> DVFFSHWTSKYKERNPTEIAYSEDIERIIDSLVTDEITKEEIIHFLFGNFCFHIETMNDQHIADKFKGYQSSCINLKIEPKVDLADLKDHLIQKQQIWESLYGKHLEKIMLRIREKKKKEKEIPDITTAFNQNAAEYEEKYPNCFTNDLSETKTNFSMTWSPSFEKIELSSEVDYNNAIINKFRESFKSSSRVIYNSPYSCINNQTNKARDITNLVRLCLTELSCDTTKMEKQELEDEIDINTGSIKVERTKKSKEWNKQGSCLTRNKNEFCMKETGRENKTIYFKGLAVMNIGMSSKKRILKKEEIKERISKGLEYDTSERQADPNDDYSSIDMSSLTHMKKLIRHDNEDSLSWCERIKDSLFVLHNGDIREEGKITSVYNNYAKNPECLYIQDSVLKTELETCKKINKLCNDLAIYHYSEDMMQFSKGLMVADRYMTKESFKILTTANTSMMLLAFKGDGMNTGGSGVPYIALHIVDEDMSDQFNICYTKEIYSYFRNGSNYIYIMRPQRLNQVRLLSLFKTPSKVPVCFAQFSKKANEMEKWLKNKDIEKVNVFSMTMTVKQILINIVFSSVMIGTVTKLSRMGIFDFMRYAGFLPLSDYSNIKEYIRDKFDPDITNVADIYFVNGIKKLLFRMEDLNLSTNAKPVVVDHENDIIGGITDLNIKCPITGSTLLTLEDLYNNVYLAIYMMPKSLHNHVHNLTSLLNVPAEWELKFRKELGFNIFEDIYPKKAMFDDKDLFSINGALNVKALSDYYLGNIENVGLMRSEIENKEDFLSPCYKISTLKSSKKCSQSNIISTDEIIECLQNAKIQDIENWKGNNLAIIKGLIRTYNEEKNRLVEFFEDNCVNSLYLVEKLKEIINSGSITVGKSVTSKFIRNNHPLTVETYLKTKLYYRNNVTVLKSKKVSEELYDLVKQFHNMMEIDLDSVMNLGKGTEGKKHTFLQMLEFVMSKAKNVTGSVDFLVSVFEKMQRTKTDREIYLMSMKVKMMLYFIEHTFKHVAQSDPSEAISISGDNKIRALSTLSLDTITSYNDILNKNSKKSRLAFLSADQSKWSASDLTYKYVLAIILNPILTTGEASLMIECILMYVKLKKVCIPTDIFLNLRKAQGTFGQNETAIGLLTKGLTTNTYPVSMNWLQGNLNYLSSVYHSCAMKAYHKTLECYKDCDFQTRWIVHSDDNATSLIASGEVDKMLTDFSSSSLPEMLFRSIEAHFKSFCITLNPKKSYASSSEVEFISERIVNGAIIPLYCRHLANCCTESSHISYFDDLMSLSIHVTMLLRKGCPNEVIPFAYGA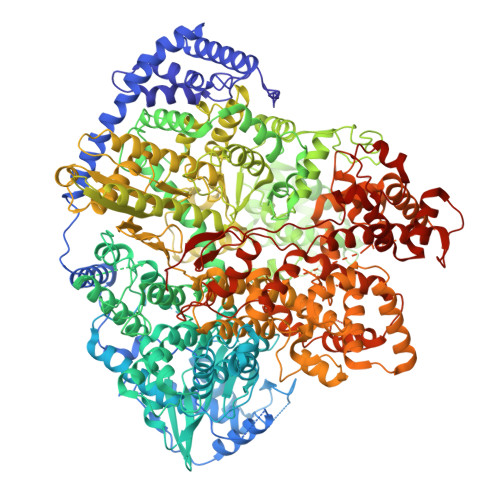VQVQALSIYSMLPGEVNDSIRIFKKLGVSLKSNEIPTNMGGWLTSPIEPLSILGPSSNDQIIYYNVIRDFLNKKSLEEVKDSVSSSSYLQMRFRELKGKYEKGTLEEKDKKMIFLINLFEKASVSEDSDVLTIGMKFQTMLTQIIKLPNFINENALNKMSSYKDFSKLYPNLKKNEDLYKSTKNLKIDEDAILEEDELYEKIASSLEMESVHDIMIKNPETILIAPLNDRDFLLSQLFMYTSPSKRNQLSNQSTEKLALDRVLRSKARTFVDISSTVKMTYEENMEKKILEMLKFDLDSYCSFKTCVNLVIKDVNFSMLIPILDSAYPCESRKRDNYNFRWFQTEKWIPVVEGSPGLVVMHAVYGSNYIENLGLKNIPLTDDSINVLTSTFGTGLIMEDVKSLVKGKDSFETEAFSNSNECQRLVKACNYMIAAQNRLLAINTCFTRKSFPFYSKFNLGRGFISNTLALLSTIYSKEES> MDSSSPLKTFRKDQAMEGKKEEIREHYNSIRERGRESRQRSKTINIRNANNFIKACLIRLYTKRGDSVLDLGCGKGGDLLKYERAGIGEYYGVDIAEVSINDARVRARNMKRRFKVFFRAQDSYGRHMDLGKEFDVISSQFSFHYAFST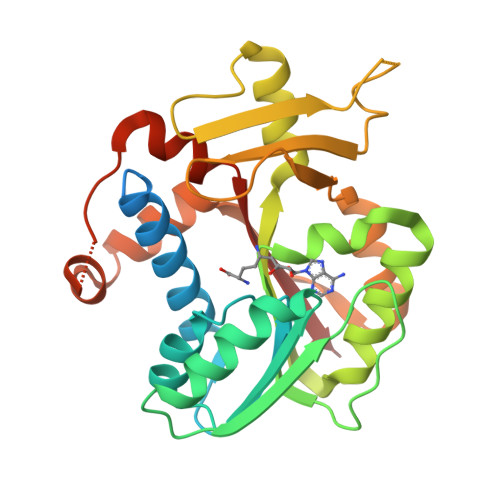SESLDIAQRNIARHLRPGGYFIMTVPSRDVILERYKQGRMSNDFYKIELEKMEDVPMESVREYRFTLLDSVNNCIEYFVDFTRMVDGFKRLGLSLVERKGFIDFYEDEGRRNPELSKKMGLGCLTREESEVVGIYEVVVFRKLVPESDA>[4x]MRGSHHHHHHGSAHGLTDDMTMHFRMEGCVDGHKFV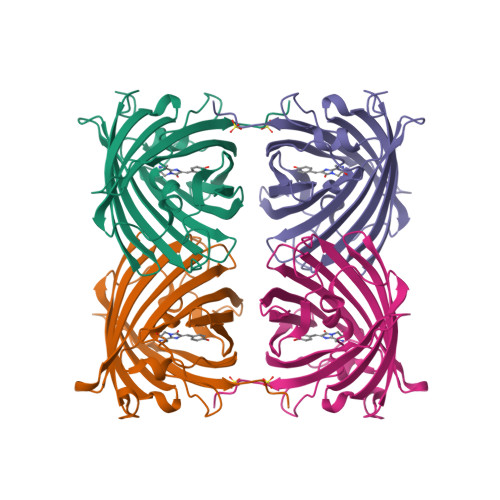IEGNGNGNPFKGKQFINLCVIEGGPLPFSEDILSAAFDYGNRLFTEYPEGIVDYFKNSCPAGYTWHRSFRFEDGAVCICSADITVNVRENCIYHESTFYGVNFPADGPVMKKMTTNWEPSCEKIIPINSQKILKGDVSMYLLLKDGGRYRCQFDTIYKAKTEPKEMPDWHFIQHKLNREDRSDAKNQKWQLIEHAIASRSALP>GARASVLSGGELDKWEKIRLRPGGKKQYKLKHIVWASRELERFAVNPGLLETSEGCRQILGQLQPSLQTGSEELRSLYNTIAVLYCVH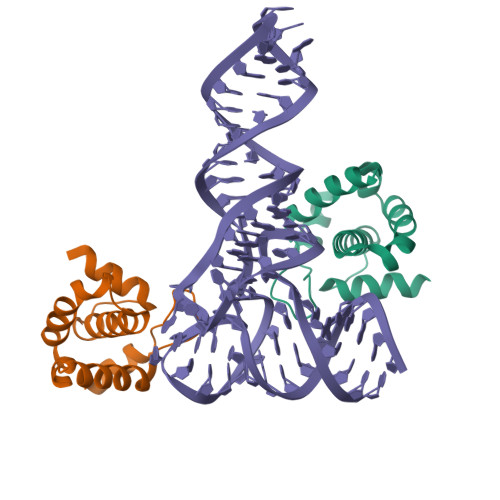QRIDVKDTKEALDKIEEEQN[2x]> QEMEGNGPAAVHYQPASPPRDACVYSSCYSEENVWKLCEYIKNHDQYPLEECYAVFISNERKMIPIWKQQARPGDGPVIWDYHVVLLHVSSGGQSFIYDLDTVLPFPCLFDTYVEDA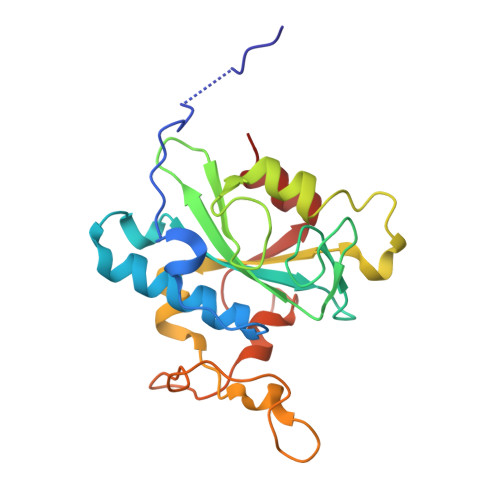IKSDDDIHPQFRRKFRVICADSYLKNFASDRSHMKDSSGNWREPPPPYPCIETGDSKMNLNDFISMDPKVGWGAVYTLSEFTHRFGS> AERSELTIHPKEFTTFVRNFNPFLGA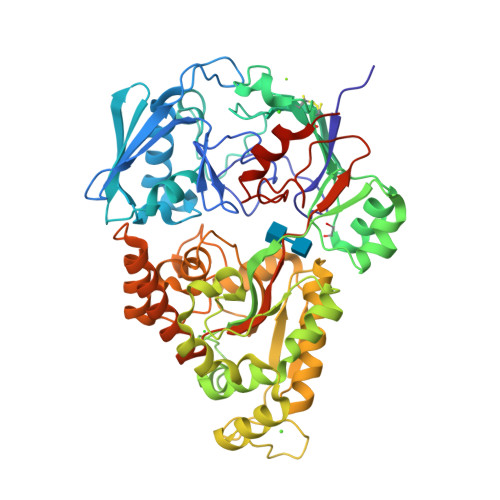TNLHTTTDFIYEPLVVFNEMHGNTPVFRLAENFQMSDDLMSVTFDIRKGVKWSDGEAFTADDVVYSFNLVKEKPELDQSGINSWVTGVEKVNDYQVKFRLSEANSNVPYEIAKVPVVPKHVWSKVKDPSTFTNENPVGSGPFTVIDTFTPQLYIQCENPNYWDAANLDVDCLRVPQIANNDQFLGKVVNGEMDWTSSFVPDIDRTYAAASPKHHYWYPPAGTQAFVVNFKNPDAAKNEALTNVDFRRAFSMALDRQTIIDIAFYGGGTVNDFASGLGYAFEAWSDEKTHDKFKAYNSYNAEGAKKLLAKAGFKDVNKDGFVDTPSGKSFELLIQSPNGATDFNNTVQLAVEQLAEVGIKARARTPDFSVYNQAMLEGTYDVAYTNYFHGADPYTYWNSAYNSALQSGDGMPRFAMHFYKNEKLDGLLNSFYKTADKQEQLEIAHGIQQIIAQDQVTIPVLSGAYMYQYNTTRFTGWWNEENPKGRPNIWAGIPERLLHVLDLKPVKLEHHHHHH>GPRTQPAENESTPIQQLLEHFLRQLQRKDPHGFFAFPVTDAIAPGYSMIIKHPMDFGTMKDKIVANEYKSVTEFKADFKLMCDNAMTYNRPDTVYYKLAKKILHAGFKMMSKQ[2x]

Bromodomain-containing protein 9 (BRD9), an essential component of the SWI/SNF chromatin remodeling complex termed ncBAF, has been established as a therapeutic target in a subset of sarcomas and leukemias. In particular, the bromodomain-containing protein 9 (BRD9), a specific component of the non-canonical (nc-BAF/GBAF) mammalian SWI/SNF chromatin remodeling complex, is essential to maintain the transformed phenotype of AML. Therefore while the BAF complexes regulate key steps in chromatin transactions required for cell fate decisions, including transcription factor binding and gene expression, the BRD9-containing BAF complex appears to play key roles in myeloid leukemia.. Paradoxically, the bromodomain in BRD9 has been shown to be an ineffectual drug target and degradation is required to reproduce the dependency seen with shRNA and CRISPR screens.

In this report, we describe a novel BRD9 bromodomain inhibitor, EA-89-YM35 (or EA-89), and a degrader-based analog (QA-68-ZU81, or QA-68) that incorporates the EA-89 warhead into a cereblon (CRBN)-targeting proteolysis-targeting chimera (PROTAC), to compare the efficacy of inhibition versus degradation to the impact seen with BRD9 knock-down (KD) by RNA interference. EA-89 is a potent and selective inhibitor that binds to BRD9 in a novel way. The binding mode of EA-89 determined by X-ray crystallography reveals that the thienopyridone head group binds to the acetyl lysine pocket similar to other known bromodomain chemotypes, forming a direct hydrogen bond with the conserved Asn100. Propyl substitution off the pyridone nitrogen accesses an adjacent induced hydrophobic pocket while the tetrahydro-2H-thiopyran ring picks up additional protein interactions, not observed with previous BI-based PROTACs, on the opposite side of the acetyl lysine pocket. X-ray co-crystal shows binding mode of EA-89 on BRD9 at 1.76 Angstroms making extended interactions across the surface of BRD9 with thienopyridone docking into the acetyl lysine pocket. HCT116 (colorectal cancer) was included as an out-of-lineage control, and JQ1, an established potent inhibitor of BET family proteins BRD2, 3, 4, was included as an inhibitor of bromodomain proteins with a distinct selectivity profile. The inhibitor, EA-89, (structure shown in Fig. 1A) produces a strongly selective profile across a subset of leukemia lines with no impact on the viability of THP-1, HEL, or HCT116. Interestingly, the degrader, QA-68, provides an >100-fold increase in potency over EA-89 and robustly degrades BRD9 in AML cells. We observed BRD9 degraders to induce differentiation of SKM-1 cells, in contrast to the BRD9 inhibitor, EA-89, which had little effect on SKM-1 differentiation and was less potent in inhibiting cell proliferation. As was observed with AML, the BRD9 degraders, QA-68 and dBRD9-A, showed higher potency against the B- ALL lines than the BRD9 inhibitor, EA-89.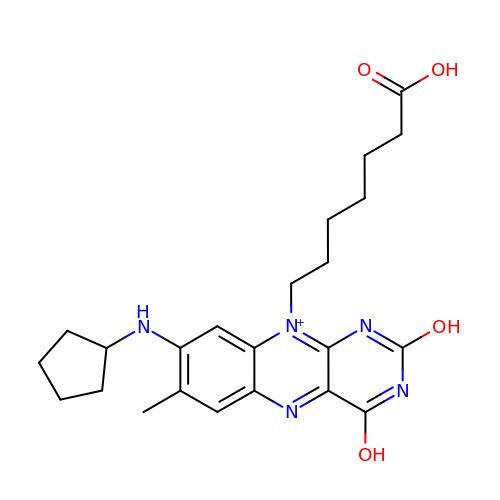10-(6-carboxyhexyl)-8-(cyclopentylamino)-2,4-dihydroxy-7-methylbenzo[g]pteridin-10-ium | C23 H30 N5 O4 | AJTKEKBUVMMJJR-UHFFFAOYSA-O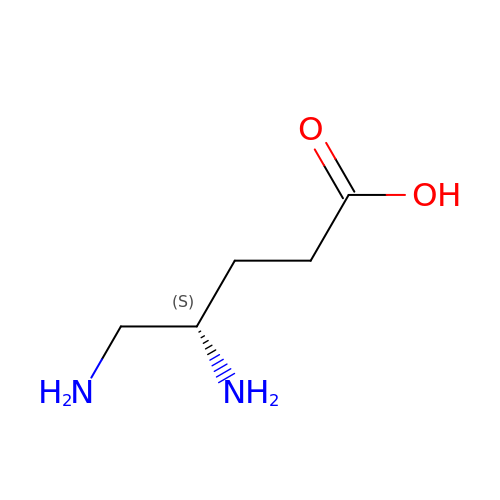(4S)-4,5-DIAMINOPENTANOIC ACID | C5 H12 N2 O2 | PQGAAJQIFBEYSA-BYPYZUCNSA-N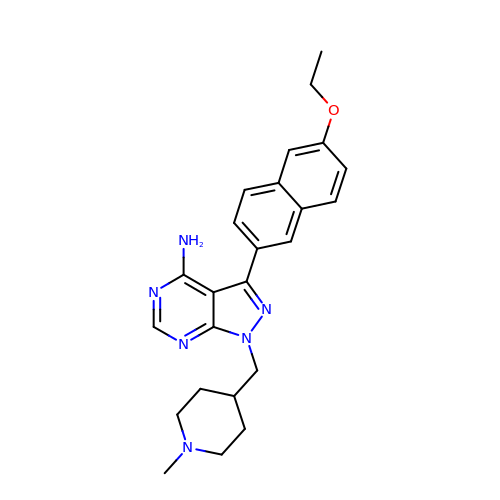3-(6-ethoxynaphthalen-2-yl)-1-[(1-methylpiperidin-4-yl)methyl]-1H-pyrazolo[3,4-d]pyrimidin-4-amine | C24 H28 N6 O | KONPIFGGWNMOKY-UHFFFAOYSA-N>[2x]GPLGSGVGNGDDEAAELMQQVNVLKLTVEDLEKERDFYFGKLRNIELI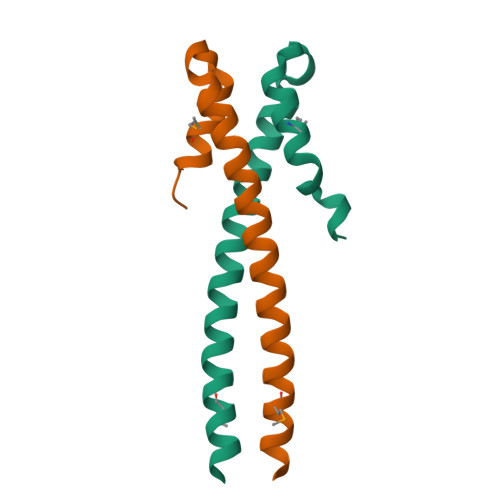CQENEGENDPVLQRIMDILYATDEGFVI>[2x]MERAESSSTEPAKAIKPIDRKSVHQICSGQVVLSLSTAVKELVENSLDAGATNIDLKLKDYGVDLIEVSDNGCGVEEENFEGLTLKHHTSKIQEFADLTQVETFGFRGEALSSLCALSDVTISTCHASAKVGTRLMFDHNGKIIQKTPYPRPRGTTVSVQQLFSTLPVRHKEFQRNIKKEYAKMVQVLHAYCIISAGIRVSCTNQLGQGKRQPVVCTGGSPSI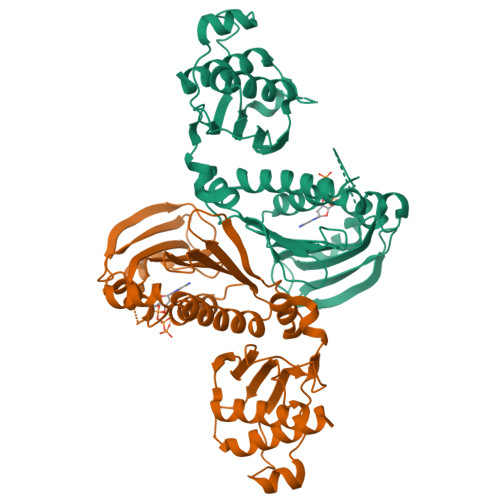KENIGSVFGQKQLQSLIPFVQLPPSDSVCEEYGLSCSDALHNLFYISGFISQCTHGVGRSSTDRQFFFINRRPCDPAKVCRLVNEVYHMYNRHQYPFVVLNISVDSECVDINVTPDKRQILLQEEKLLLAVLKTSLIGMFDS> PGSVVELLGKSYPQDDHSNLTRKVLTRVGRNLHNQQHHPLWLIKERVKEHFYKQYVGRFGTPLFSVYDNLSPVVTTWQNFDSLLIPADHPSRKKGDNYYLNRTHMLRAHTSAHQWDLLHAGLDAFLVVGDVYRRDQIDSQHYPIFHQLEAVRLFSKHELFAGIKDGESLQLFEQSSRSAHKQETHTMEAVKLVEFDLKQTLTRLMAHLFGDELEIRWVDCYFPFTHPSFEMEINFHGEWLEVLGCGVMEQQLVNSAGAQDRIGWAFGLGLERLAMILYYIPDIRLFWCEDERFLKQFCVSNINQKVKFQPLSKYPAVINDISFWLPSENYAENDFYDLVRTIGGDLVEKVDLID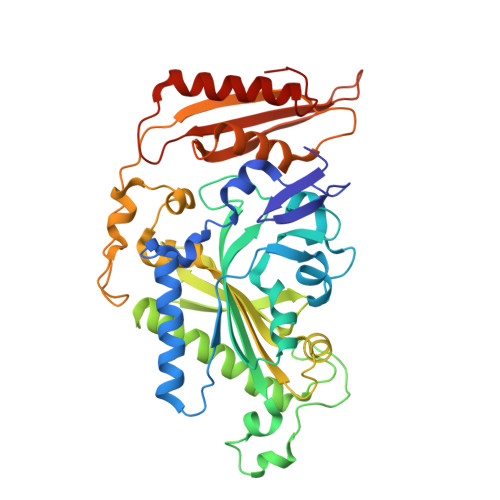KFVHPKTHKTSHCYRITYRHMERTLSQREVRHIHQALQEAAVQLLGVEGRF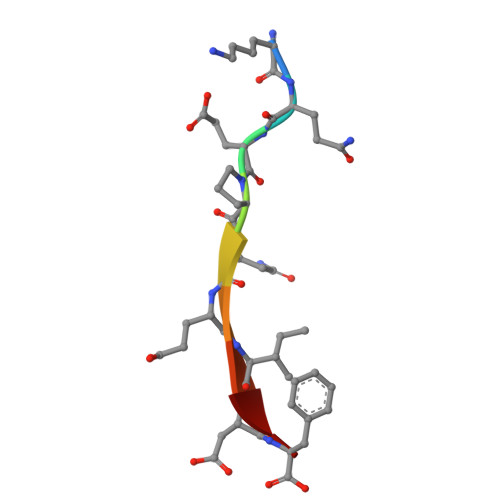> KQEPQEIDF>MIVLFVDFDYFYAQVEEVLNPSLKGKPVVVCVFSGRFEDSGAVATANYEARKFGVKAGIPIVEAKKILPNAVYLPMRKEVYQQVSSRIMNLLREYSEKIEIASIDEAYLDISDKVRDYREAYNLGLEIKNKILEKEKITVTVGISKNKVFAKIAADMAKPNGIKVIDDEEVKRLIRELDIADVPGIGNITAEKLKKLGINKLVDTLSIEFDKLKGMIGEAKAKYLISLARDEYNEPIRTRVRKSIGRIVTMKRNSRNLEEIKPYLFRAIEESYYKLDKRIPKAIHVV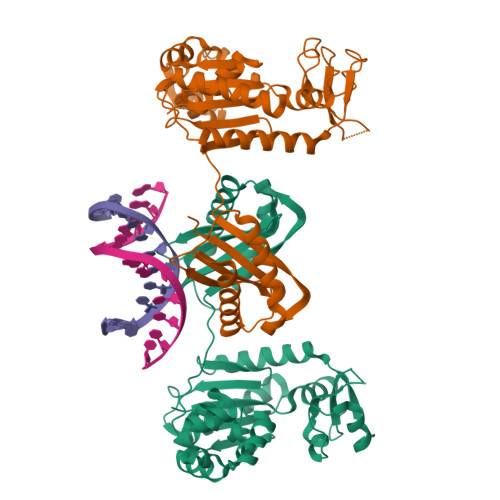AVTEDLDIVSRGRTFPHGISKETAYSESVKLLQKILEEDERKIRRIGVRFSKFIEAIGLDKFFDTLEHHHHHH[2x]> MVLERNETMYYGGSLWSPPSNWNPFTPWNAVPGTTGLVYETMFFYDPLTGNFDPWLAEKGEWLDSKTYRVVLREGIYWHDNVPLTSEDVRFTFEIAKKYKGIHYSSVWEWLDHIETPDNRTVIFVFKDPRYHEWNELLYTLPIVPKHIWEEKDETTILQSSNEYPLGSGPYVAHSWDQNKMIFERFENWWGTKVMGVKPAPKYVVIVRVLSNNVALGMLMKGELDFSNFMLPGVPILKKVYNLNTWYDEPPYHLSSTVVGLFLNARKYPLSLPEFRRAIAMSINADPIVQRVYEGAVLKADPLGFLPNSVWMKYYPKEVVEKHGFKYDPEEAKSILDKLGFRDVNGDGFRETPDGKPIKLTIECPYGWTDWMQAIQ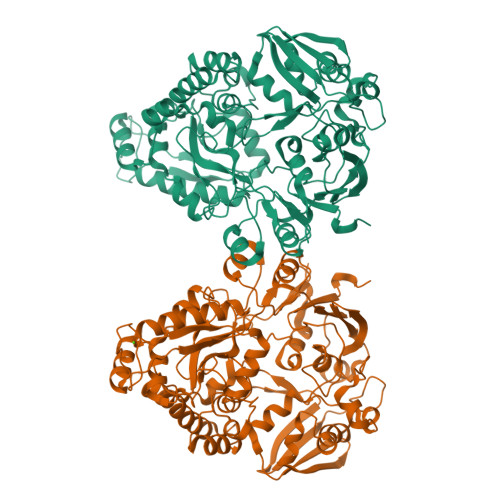VIVDQLKVVGINAEPYFPDSSKYYENMYKGEFDIEMNANGTGISSTPWTYFNTIFYPDALESEFSYTGNYGRYQNPEVESLLEELNRTPLDNVEKVTELCGKLGEILLKDLPFIPLWYGAMAFITQDNVWTNWPNEHNPYAWPCGWANWWQTGALKILFNLKPAKHHHHHH>[3x]MSEQFQMTRRSMLAGAAIAGAVTPLI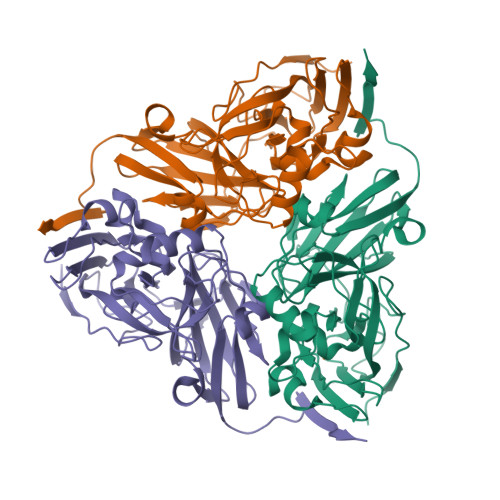GAVSAHAEEAVAKTAHINVASLPRVKVDLVKPPFVHAHTQKAEGGPKVVEFTLTIEEKKIVIDEQGTELHAMTFNGSVPGPLMVVHQDDYVELTLINPDTNTLQHNIDFHSATGALGGGALTVVNPGDTTVLRFKASKAGVFVYHCAPPGMVPWHVTSGMNGAIMVLPREGLTDGKGNSITYDKVYYVGEQDFYVPRDANGKFKKYESVGEAYADTLEVMRTLTPSHIVFNGAVGALTGDSALKAAVGEKVLIVHSQANRDTRPHLIGGHGDYVWATGKFRNAPDVDQETWFIPGGTAGAAFYTFEQPGIYAYVNHNLIEAFELGAAAHFAVTGDWNDDLMTSVRAPSGT> 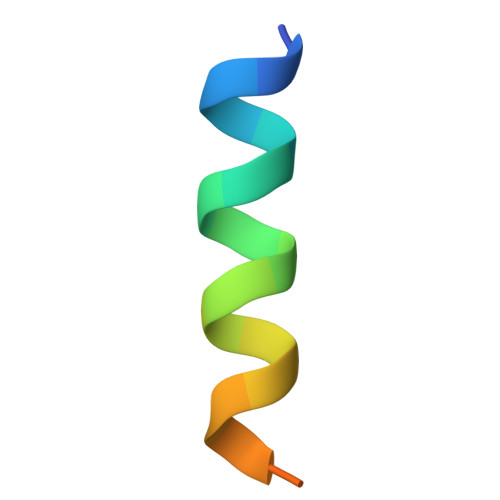ALEEDAQILKVIEAYCTSAKT>MATSGFSKPLHYPPVRRDETVVDDYFGVKVADPYRWLEDPNSEETKEFVDNQEKLANSVLEECELIDKFKQKIIDFVNFPRCGVPFRRANKYFHFYNSGLQAQNVFQMQDDLDGKPEVLYDPNLREGGRSGLSLYSVSEDAKYFAFGIHSGLTEWVTIKILKTEDRSYLPDTLEWVKFSPAIWTHDNKGFFYCPYPPLKEGEDHMTRSAVNQEARYHFLGTDQSEDILLWRDLENPAHHLKCQITDDGKYFLLYILDGCDDANKVYCLDLTKLPNGLESFRGREDSAPFMKLIDSFDASYTAIANDGSVFTFQTNKDAPRKKLVRVDLNNPSVWTDLVPESKKDLLESAHAVNENQLILRYLSDVKHVLEIRDLESGALQHRLPIDIGSVDGITARRRDSVVFFKFTSILTPGIVYQCDLKNDPTQLKIFRESVVPDFDRSEFEVKQVFVPSKDGTKIPIFIAARKGISLDGSHPCEMHGYGGFGINMMPTFSASRIVFLKHLGGVFCLANIRG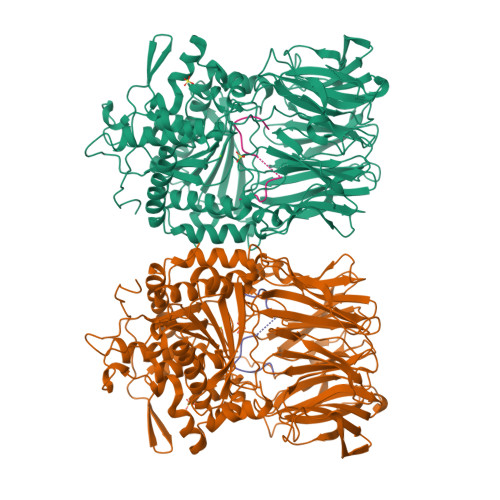GGEYGEEWHKAGFRDKKQNVFDDFISAAEYLISSGYTKARRVAIEGGANGGLLVAACINQRPDLFGCAEANCGVMDMLRFHKFTLGYLWTGDYGCSDKEEEFKWLIKYSPIHNVRRPWEQPGNEETQYPATMILTADHDDRVVPLHSFKLLATMQHVLCTSLEDSPQKNPIIARIQRKAAHYGRATMTQIAEVADRYGFMAKALEAPWID[2x];>MSPILAHDVVKPQGVAWAFQAKDVENASAPV[2x]> VDMFLYNLTLQRATGISFAIHGNFSGTKQQEIVVSRGKILELLRPDPNTGKVHTLLTVEVFGVIRSLMAFRLTGGTKDYIVVGSDSGRIVILEYQPSKNMFEKIHQETFGKSGCRRIVPGQFLAVDPKGRAVMISAIEKQKLVYILNRDAAARLTISSPLEAHKANTLVYHVVGVDVGFENPMFACLEMDYEEADNDPTGEAAANTQQTLTFYELDLGLNHVVRKYSEPLEEHGNFLITVPGGSDGPSGVLICSENYITYKNFGDQPDIRCPIPRRRNDLDDPERGMIFVCSATHKTKSMFFFLAQTEQGDIFKITLETDEDMVTEIRLKYFDTVPVAAAMCVLKTGFLFVASEFGNHYLYQIAHLGDDDEEPEFSSAMPLEEGDTFFFQPRPLKNLVLVDELDSLSPILFCQIADLANEDTPQLYVACGRGPRSSLRVLRHGLEVSEMAVSELPGNPNAVWTVRRHIEDEFDAYIIVSFVNATLVLSIGETVEEVTDSGFLGTTPTLSCSLLGDDALVQVYPDGIRHIRADKRVNEWKTPGKKTIVKCAVNQRQVVIALTGGELVYFEMDPSGQLNEYTERKEMSADVVCMSLANVPPGEQRSRFLAVGLVDNTVRIISLDPSDCLQPLSMQALPAQPESLCIVEMGGTEKQDELGERGSIGFLYLNIGLQNGVLLRTVLDPVTGDLSDTRTRYLGSRPVKLFRVRMQGQEAVLAMSSRSWLSYSYQSRFHLTPLSYETLEFASGFASEQCPEGIVAISTNTLRILALEKLGAVFNQVAFPLQYTPRKFVIHPESNNLIIIETDHNAYTEATKAQRKQQMAEEMVEAAGEDERELAAEMAAAFLNENLPESIFGAPKAGNGQWASVIRVMNPIQGNTLDLVQLEQN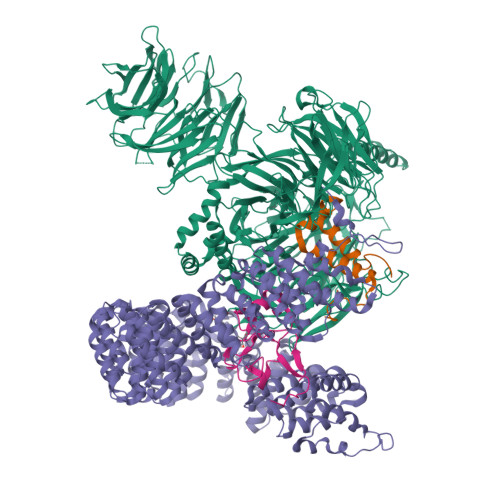EAAFSVAVCRFSNTGEDWYVLVGVAKDLILNPRSVAGGFVYTYKLVNNGEKLEFLHKTPVEEVPAAIAPFQGRVLIGVGKLLRVYDLGKKKLLRKCENKHIANYISGIQTIGHRVIVSDVQESFIWVRYKRNENQLIIFADDTYPRWVTTASLLDYDTVAGADKFGNICVVRLPPNTNDEVDSQKAEVIMNYHVGETVLSLQKTTLIPGGSESLVYTTLSGGIGILVPFTSHEDHDFFQHVEMHLRSEHPPLCGRDHLSFRSYYFPVKNVIDGDLCEQFNSMEPNKQKNVSEELDRTPPEVSKKLEDIRTRYAFDYKDDDDK;> TDRYTIHSQLEHLQSKYIGTGHADTTKWEWLVNQHRDSYCSYMGHFDLLNYFAIAENESKARVRFNLMEKMLQPCGPPADKPEEN;> MKSVNDQPSGNLPFLKPDDIQYFDKLLVDVDESTLSPEEQKERKIMKLLLKIKNGTPPMRKAALRQITDKAREFGAGPLFNQILPLLMSPTLEDQERHLLVKVIDRILYKLDDLVRPYVHKILVVIEPLLIDEDYYARVEGREIISNLAKAAGLATMISTMRPDIDNMDEYVRNTTARAFAVVASALGIPSLLPFLKAVCKSKKSWQARHTGIKIVQQIAILMGCAILPHLRSLVEIIEHGLVDEQQKVRTISALAIAALAEAATPYGIESFDSVLKPLWKGIRQHRGKGLAAFLKAIGYLIPLMDAEYANYYTREVMLILIREFQSPDEEMKKIVLKVVKQCCGTDGVEANYIKTEILPPFFKHFWQHRMALDRRNYRQLVDTTVELANKVGAAEIISRIVDDLKDEAEQYRKMVMETIEKIMGNLGAADIDHKLEEQLIDGILYAFQEQTTEDSVMLNGFGTVVNALGKRVKPYLPQICGTVLWRLNNKSAKVRQQAADLISRTAVVMKTCQEEKLMGHLGVVLYEYLGEEYPEVLGSILGALKAIVNVIGMHKMTPPIKDLLPRLTPILKNRHEKVQENCIDLVGRIADRGAEYVSAREWMRICFELLELLKAHKKAIRRATVNTFGYIAKAIGPHDVLATLLNNLKVQERQNRVCTTVAIAIVAETCSPFTVLPALMNEYRVPELNVQNGVLKSLSFLFEYIGEMGKDYIYAVTPLLEDALMDRDLVHRQTASAVVQHMSLGVYGFGCEDSLNHLLNYVWPNVFETSPHVIQAVMGALEGLRVAIGPCRMLQYCLQGLFHPARKVRDVYWKIYNSIYIGSQDALIAHYPRIYNDDKNTYIRYELDYIL;> GPLGSPGSRAMAKHHPDLIFCRKQAGVAIGRLCEKCDGKCVICDSYVRPCTLVRICDECNYGSYQGRCVICGGPGVSDAYYCKECTIQEKDRDGCPKIVNLGSSKTDL> PLTEQEIDELCDEWVPEPLIPPITEDMKHEPPVLESAAGPHTTVNGKDVVNFASANYLGLIGHEKLLESCTSALEKYGVGSCGPRGFYGTIDVHLDCETRISKFLGTPDSILYSYGLSTMFSTIPCFCKKGDVIVADEGVHWGIQNGLQLSRSTIVYFKHNDMESLRITLEKIMTKYKRSKNLRRYIVAEAVYQNSGQIAPLDEIVKLKEKYRFRVILDESNSFGVLGRSGRGLAEHHSVPIEKID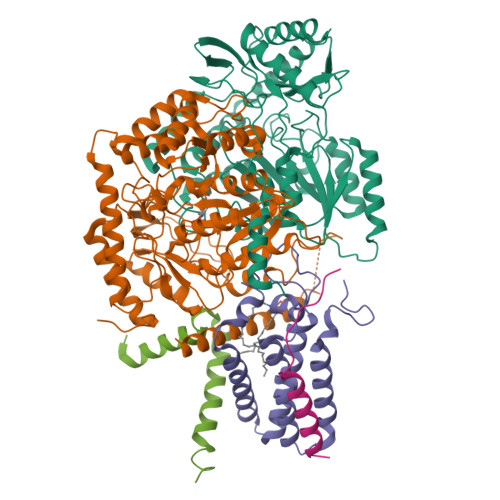VVTAAMGHALATEGGFCTGNARIIDYQRLSSSGYVFSASLPPYLASAAITAIDVIDQNPDMLVKLKQNVALLWKGLSDIKGMSLTSNRESPIVFLKLEKSSGSAKDDLLLLEKMADRALKEDSLLVVSSKRSFLDKCRLPVGIKLYVSAGHSESDLLKASESLKRLASELLLKS;> MYLTAVSTYFSYGLLFAFGQLRDFFRRFIDWWFTSNLQGYAPICLGHEDFYIRRLYHRIQDCFERPISSAPDAWFDVVERYSNDNNKTLKRTTKTSRCLNLGSYNYLGFGSFDEYCTPRVIESLKKFSASTCSSRVDAGTTSVHAELEECVTRFVGKPAAVVFGMGYATNSAIIPVLIGKGGLIISDSLNHSSIVNGARGSGATIRVFQHNTPSHLERVLREQIAEGQPRTHRPWKKIIVVVEGIYSMEGEICHLPEVVAICKKYKAYVYLDEAHSIGAIGKTGKGICELLGVDTADVDVMMGTFTKSFGSCGGYIAGSKELIQYLKHQCPAHLYATSIPTPSAQQIISAIKVILGEDGSNRGAQKLARIRENSNFFRAELQKMGFEVLGDNDSPVMPIMLYNPAKIPAFSRECLRQKVAVVVVGFPATPLLLARARICISASHSREDLIRALKVISKVGDLSGIKYFPAEPKKIEQSKNDIKLD;> MADYKDDDDKSGPDEVDASGRMNWVQRKIYLYNVTFGLYMLDWWERYLFNSLVVVLMWFVLYNGTRYFSELFQRHLT;> MANLYVKAVPPPDMNRNTEWFMYPGVWTTYMLILFFGWLVVLSVSGCSPGMAWTVVNLAHFVVTYHSFHWMKGTPFADDQGIYNGLTWWEQMDNGQQLTRNRKFLTLVPVVLYLIASHTTDYRHPWLFLNTLAVMVLVVAKFPNMHKVRIFGINGDK;> MASNLVEMFNAALNWVTMILESPSARVVLFGVPIRGHFFVEGLLGVVIIILLTRKSYKPPKR> MVKIVYPNAKDFFSFINSITNVTDSIILNFTEDGIFSRHLTEDKVLMAIMRIPKDVLSEYSIDSPTSVKLDVSSVKKILSKASSKKATIELTETDSGLKIIIRDEKSGAKSTIYIKAEKGQVEQLTEPKVNLAVNFTTDESVLNVIAADVTLVGEEMRISTEE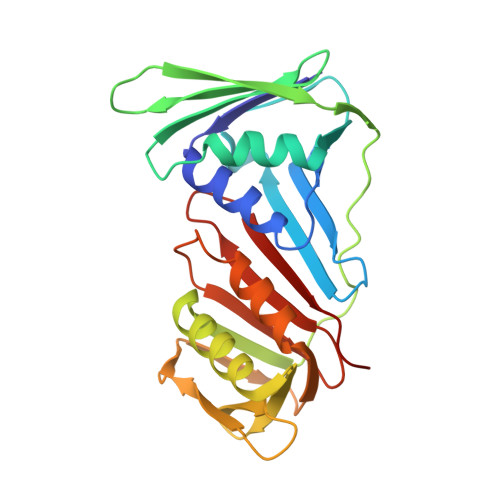DKIKIEAGEEGKRYVAFLMKDKPLKELSIDTSASSSYSAEMFKDAVKGLRGFSAPTMVSFGENLPMKIDVEAVSGGHMIFWIAPRL>DSYYQRSDWTADEEQILLGPFDYLESLPGKNMRSQLIQSFNTWLKVPTESLDVIIKVISMLHTASLLIDDIQDQSILRRGQPVAHSIFGTAQAMNSGNYVYALALREVQKLQNPKAISIYVDSLIDLHRGQGMELFWRDSLMCPTEEQYLDMVANKTGGLFCLAIQLMQAEATIQVDFIPLVRLLGIIFQICDDYLNLKSTAYTDNKGLCEDLTEGKFSFPIIHSIRSNPGNRQLINILKQKPREDDIKRYALSYMESTNS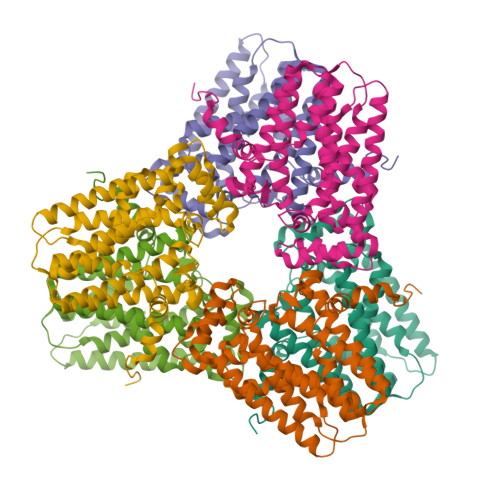FEYTRGVVRKLKTEAIDTIQGLEKHGLEENIGIRKILARMSLEL[2x]> ATSDSNMLLNYVPVYVMLPLGVVNVDNVFEDPDGLKEQLLQLRAAGVDGVMVDVWWGIIELKGPKQYDWRAYRSLLQLVQECGLTLQAIMSFHQCGGNVGDIVNIPIPQWVLDIGESNHDIFYTNRSGTRNKEYLTVGVDNEPIFHGRTAIEIYSDYMKSFRENMSDFLESGLIIDIEVGLGPAGELRYPSYPQSQGWEFPGIGEFQCYDKYLKADFKAAVARAGHPEWELPDDAGKYNDVPESTGFFKSNGTYVTEKGKFFLTWYSNKLLNHGDQILDEANKAFLGCKVKLAIKVSGIHWWYKVENHAAELTAGYYNLNDRDGYRPIARMLSRHHAILNFVCLEMRDSEQPSDAKSGPQELVQQVLSGGWREDIRVAGENALPRYDATAYNQIILNARPQGVNNNGPPKLSMFGVTYLRLSDDLLQKSNFNIFKK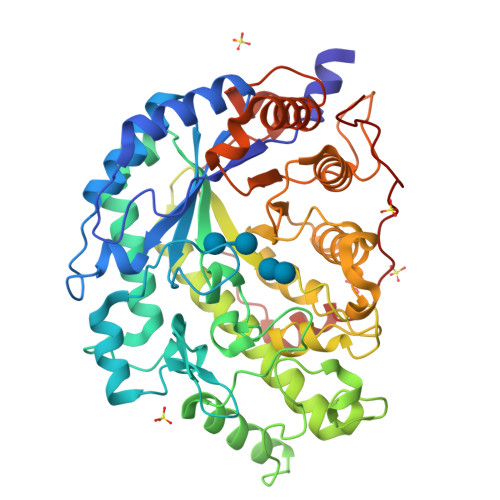FVLKMHADQDYCANPQKYNHAITPLKPSAPKIPIEVLLEATKPTLPFPWLPETDMKVDG> KQKFQSVFTVTRQTHQPPAPNSLIRFNA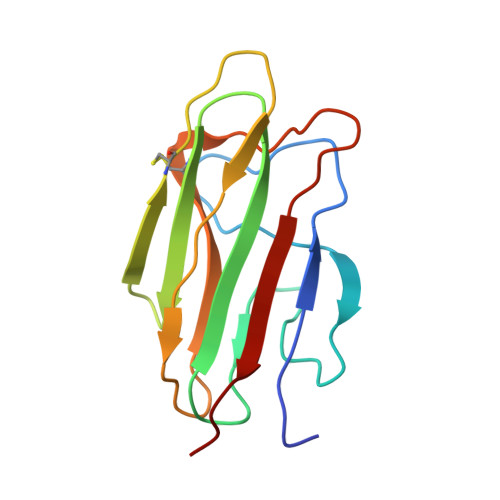VLTNPQGDYDTSTGKFTCKVPGLYYFVYHASHTANLCVLLYRSGVKVVTFCGHTSKTNQVNSGGVLLRLQVGEEVWLAVNDYYDMVGIQGSDSVFSGFLLFPD The eukaryotic translation initiation factor 4E (eIF4E) protein is a vital component of the cap-dependent mechanism for mRNA translation. It binds the 7-methylguanosine (m7G) cap structure present at the 5′ end of mRNA molecules and recruits it as part of the eIF4F assembly which also includes two other partner proteins, eIF4A and eIF4G, to the translational machinery for protein synthesis. We have used a structure-guided approach to rationally develop a set of hydrocarbon stapled-peptides with high binding affinities and residence times against the oncogenic eukaryotic translation initiation factor 4E (eIF4E) protein. Crystal structures of these peptides in complex with eIF4E show that they form specific interactions with a region on the protein-binding interface of eIF4E which is distinct from the other well-established canonical interactions.

The lifetime of binding measured in terms of the residence time (RT = 1/koff) was also found to be higher for the 13mer peptides (∼36 seconds) compared to their 12mer counterparts (10 seconds for sTIP-05 and 6 seconds for sTIP-06). Crystal structures of the complexes of sTIP-07 and sTIP-08 with eIF4E were determined (C and Table S1†). The essential interactions made by the parent 12mer peptides were retained. In the crystal structure of sTIP-08 with eIF4E, only the density for the lysine moiety (Lys) of the modified residue “Lys(ButPhI)” (&13) was visible, forming hydrophobic interactions with W73, Y76 and L131 in the patch and potentially engaging the side-chain of N77 via a hydrogen-bond. We computationally modeled the missing functional group of &13 and subjected sTIP-07 and sTIP-08 complex structures to MD simulations. The “ButPhI” functional group of residue &13 in sTIP-08 was observed to be dynamic in the simulation and did not form any stable interactions with the protein (Movie S4†). Conversely, the “Lys” chain remained largely bound to the protein surface and significantly contributed to the binding energy (–3.6 kcal mol–1) between the protein and &13 at the C-terminus. This physical association with the protein could be the primary reason for the relative stability of the moiety and hence its resolution in the crystal structure. In summary, extending the C-termini of two stapled peptides with tryptophan or effectively lysine resulted in the efficient engagement of a previously untapped patch on eIF4E and an increase in the residence time of the peptide–protein complex.

> MVANPEHYIKHPLQNRWALWFFKNDKSKTWQANLRLISKFDTVEDFWALYNHIQLSSNLMPGCDYSLFKDGIEPMWEDEKNKRGGRWLITLNKQQRRSDLDRFWLETLLCLIGESFDDYSDDVCGAVVNVRAKGDKIAIWTTECENREAVTHIGRVYKERLGLPPKIVIGYQSHADTATKSGSTTKNRFVV;> XRIIYSRLQLLLLKX> GSSRAMGNEVAGVEDISVEITPSSK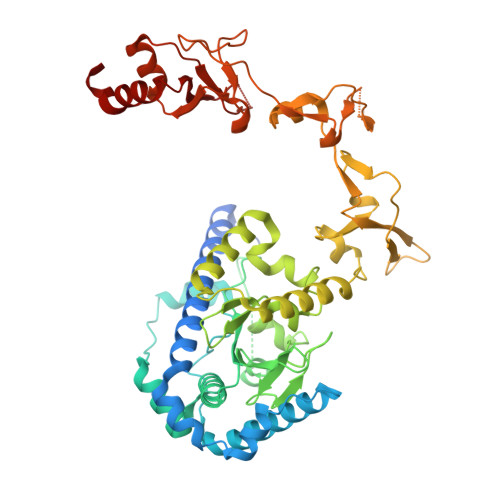RNSDARRTSRNCSSNEERKRRKYFHMLYLVCLMVHGFIRNEWINSKRLSRKLSNLVPEKVFELLHPQKDEELPLRSTRKLLDGLKKCMELWQKHWKITKKYDNEGLYMRTWKEIEMSANNKRKFKTLKRSDFLRAVSKGHGDPDISVQGFVAMLRACNVNARLIMSCQPPDFTNMKIDTSLNGNNAYKDMVKYPIFWCEVWDKFSKKWITVDPVNLKTIEQVRLHSKLAPKGVACCERNMLRYVIAYDRKYGCRDVTRRYAQWMNSKVRKRRITKDDFGEKWFRKVITALHHRKRTKIDDYEDQYFFQRDESEGIPDSVQDLKNHPYYVLEQDIKQTQIVKPGCKECGYLKVHGKVGKVLKVYAKRDIADLKSARQWYMNGRILKTGSRCKKVIKRTVGRPKGEAEEEDERLYSFEDTELYIPPLASASGEITKNTFGNIEVFAPTMIPGNCCLVENPVAIKAARFLGVEFAPAVTSFKFERGSTVKPVLSGIVVAKWLREAIETAIDGIEFI2-[[2-methyl-3-(trifluoromethyl)phenyl]amino]pyridine-3-carboxylic 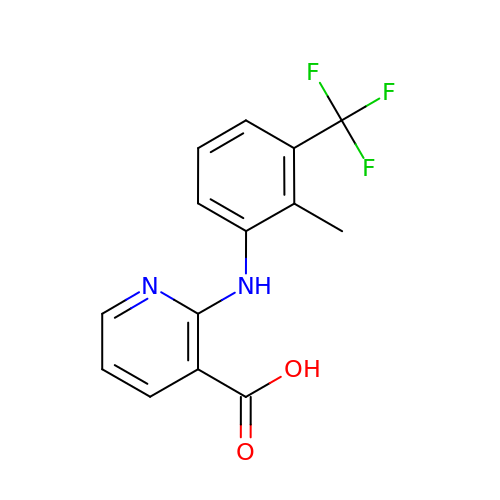acid | C14 H11 F3 N2 O2 | NOOCSNJCXJYGPE-UHFFFAOYSA-N> 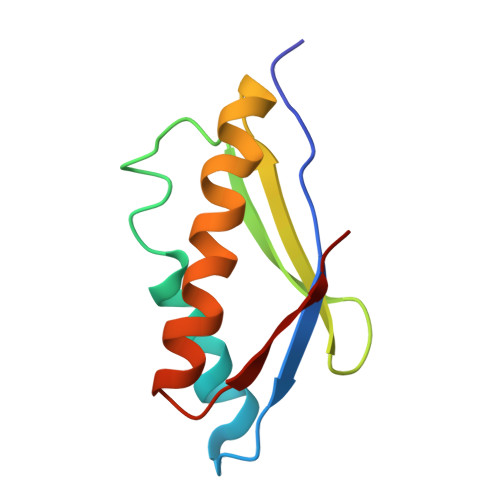MRKVKMSGLITVRTNEPLGVEKIKEVISKALENIEQDYESLLNIKIYTIGAPRYRVDVVGTNPKEASEALNQIISNLIKIGKEENVDISVVKK3'-1-CARBOXY-1-PHOSPHONOOXY-ETHOXY-URIDINE-DIPHOSPHATE-N-ACETYLGLUCOSAMINE | C20 H32 N3 O23 P3 | 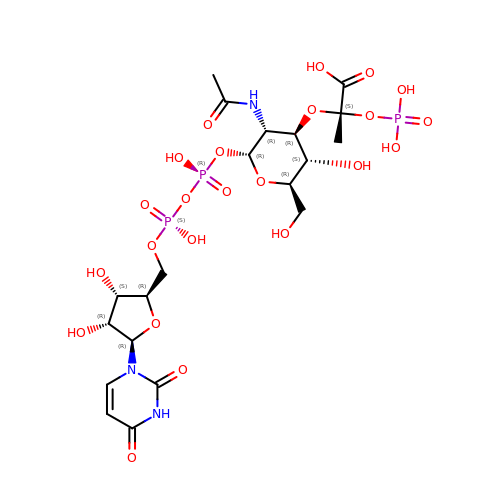NLBIPGBVVPCESQ-BVDGEXFOSA-N>GHMEQTARAIFRFVPRHEDELE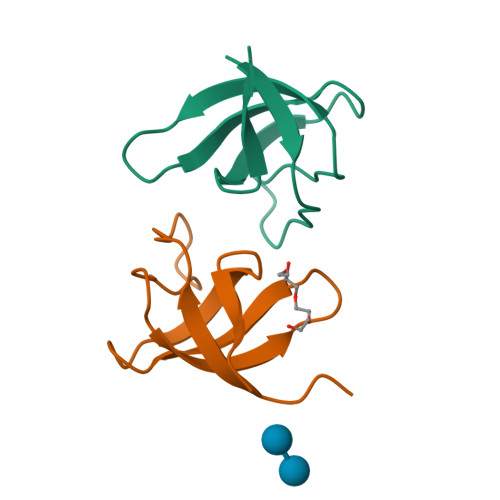LEVDDPLLVELQAEDYWYEAYNMRTGARGVFPAYYAIEVTK[2x]>[6x]PPGPPGPP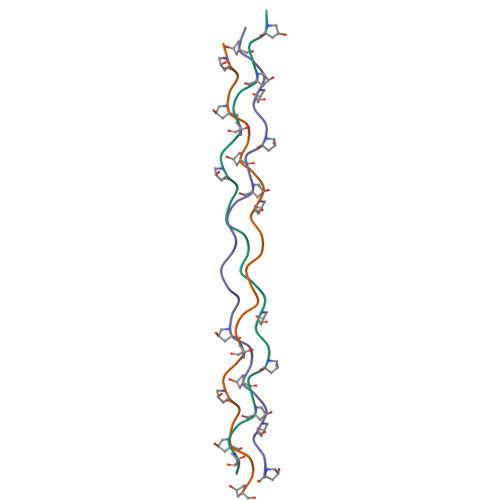GPPGPKGDQGPPGPPGPPGPPG>MVGEEKMSLRNRLSKSRENPEEDEDQRNPAKESLETPSNGRIDI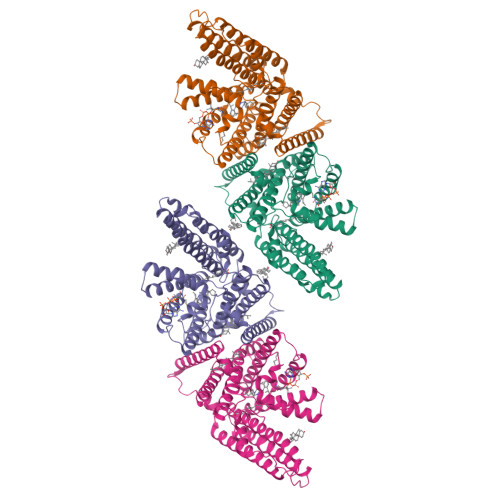KQLIAKKIKLTAEAEELKPFFMKEVGSHFDDFVTNLIEKSASLDNGGCALTTFSVLEGEKNNHRAKDLRAPPEQGKIFIARRSLLDELLEVDHIRTIYHMFIALLILFILSTLVVDYIDEGRLVLEFSLLSYAFGKFPTVVWTWWIMFLSTFSVPYFLFQHWATGYSKSSHPLIRSLFHGFLFMIFQIGVLGFGPTYVVLAYTLPPASRFIIIFEQIRFVMKAHSFVRENVPRVLNSAKEKSSTVPIPTVNQYLYFLFAPTLIYRDSYPRNPTVRWGYVAMKFAQVFGCFFYVYYIFERLCAPLFRNIKQEPFSARVLVLCVFNSILPGVLILFLTFFAFLHCWLNAFAEMLRFGDRMFYKDWWNSTSYSNYYRTWNVVVHDWLYYYAYKDFLWFFSKRFKSAAMLAVFAVSAVVHEYALAVCLSFFYPVLFVLFMFFGMAFNFIVNDSRKKPIWNVLMWTSLFLGNGVLLCFYSQEWYARQHCPLKNPTFLDYVRPRSWTCRYVFDYKDDDDK[4x]>MSTKQHSAKDELLYLNKAVVFGSGAFGTALAMVLSKKCREVCVWHMNEEEVRLVNEKRENVLFLKGVQLASNITFTSDVEKAYNGAEIILFVIPTQFLRGFFEKSGGNLIAYAKEKQVPVLVCTKGIERSTLKFPAEIIGEFLPSPLLSVLAGPSFAIEVATGVFTCVSIASADINVARRLQRIMSTGDRSFVCWATTDTVGCEVASAVKNVLAIGSGVANGLGMGLNARAALIMRGLLEIRDLTAALGGDGSAVFGLAGLGDLQLTCSSELSRNFTVGKK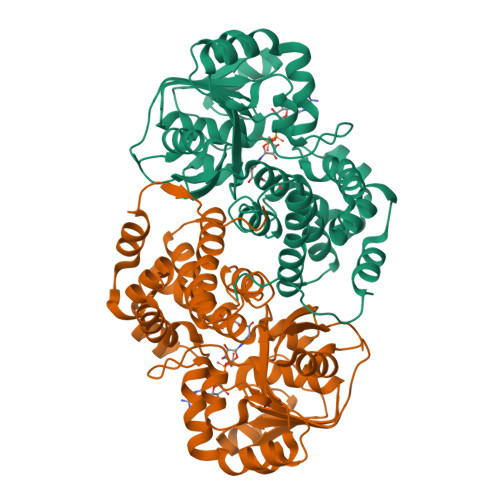LGKGLPIEEIQRTSKAVAEGVATADPLMRLAKQLKVKMPLCHQIYEIVYKKKNPRDALADLLSCGLQDEGLPPLFKRSASTPSKL[2x]> QEL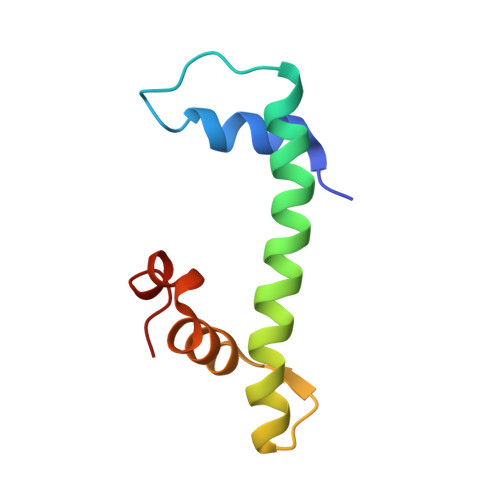PLARIKKIMKLDEDVKMISAEAPVLFAKAAQIFITELTLRAWIHTEDNKRRTLQRNDIAMAITKFDQFDFLIDIVPR>[9x]MTENIPLRVQFKRMSADEWARSDVILLEGEIGFETDTGFAKFGDGQNTFSKLKYLTGPKGPKGDTGLQGKTGGTGPRGPAGKPGTTDYDQLQNKPDLGAFAQKEETNSKITKLESSKADKSAVYSKAESKIELDKKLSLTGGIVTGQLQFKPNKSGIKPSSSVGGAINIDMSKSEGAAMVMYTNKDTTDGPLMILRSDKDTFDQSAQFVDYSGKTNAVNIVMRQPSAPNFSS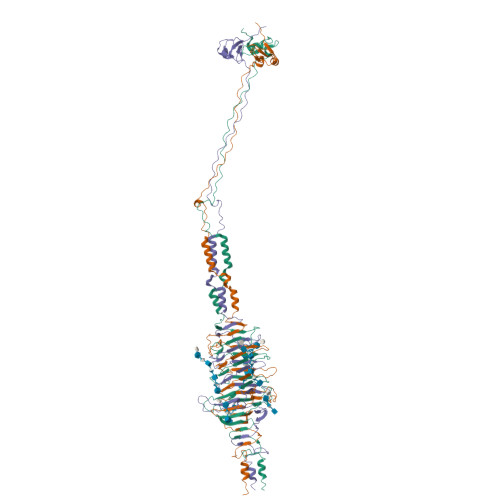ALNITSANEGGSAMQIRGVEKALGTLKITHENPNVEAKYDENAAALSIDIVKKQKGGKGTAAQGIYINSTSGTAGKMLRIRNKNEDKFYVGPDGGFHSGANSTVAGNLTVKDPTSGKHAATKDYVDEKIAELKKLILKKLEHHHHHH>GASGDVCQDCIQMVTDIQTAVRTNSTFVQALVEHVKEECDRLGPGMADICKNYISQYSEIAIQMMMHMQPKEICALVGFCDE[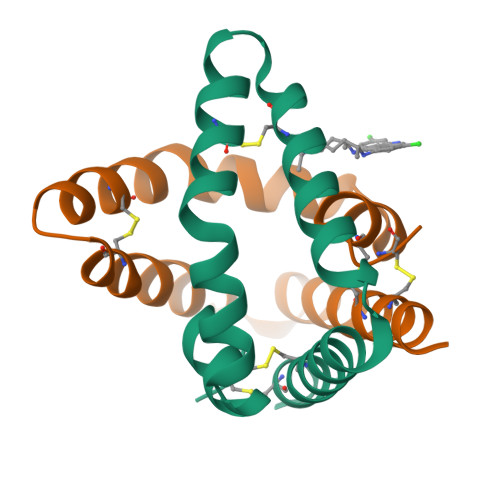3x]> RHFEETDDAYVAGNQIQIMSQVSGSVTKVWADNTDFVKEGDVLVTLDPTDARQAFEKAKTALASSVRQTHQLMINSKQLQANIEVQKIALAKAQSDYNRRVPLGNANLIGREELQHARDAVTSAQAQLDVAIQQYNANQAMILGTKLEDQPAVQQAATEVRNAWLALERTRIISPMTGYVSRRAVQPGAQISPTTPLMAVVPATNMWVDANFKETQIANMRIGQPVTITTDIYGDDVKYTGKVVGLDMGTGSAFSLLPAQNATGNWIKVVQRLPVRIELDQKQLEQYPLRIGLSTLVSVNTTNRD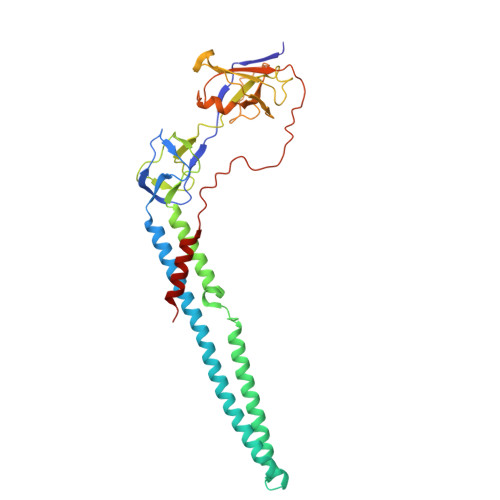GQVLANKVRSTPVAVSTAREISLAPVNKLIDDIVKANAG>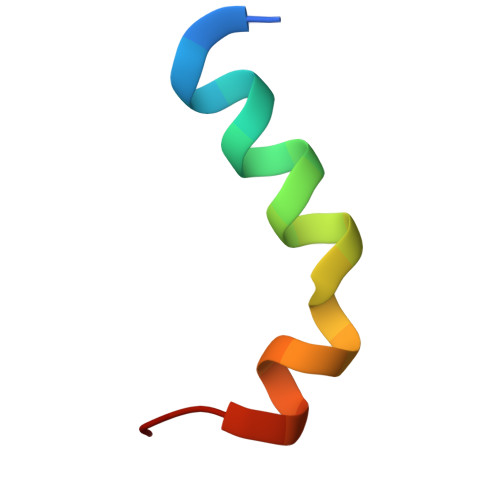 RRDYTEQLRRAARRNAWDLYGEHFY>MPTQLEMAMDTMIRIFHRYSGKERKRFKLSKGELKLLLQRELTEFLSCQKETQLVDKIVQDLDANKDNEVDFNEFVVMV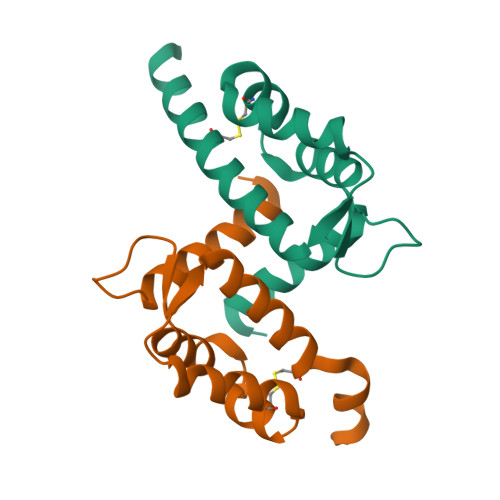AALTVACNDYFVEQLKKKGK[4x]>KKKGSVVIVGRINLSGDTAYAQQTRGEEGCQETSQTGRDKNQVEGEVQIVSTATQTFLATSINGVLWTVYHGAGTRTIASPKGPVTQMYTNVDKDLVGWQAPQGSRSLTPCTCGSSDLYLVTRHADVIPVRRRG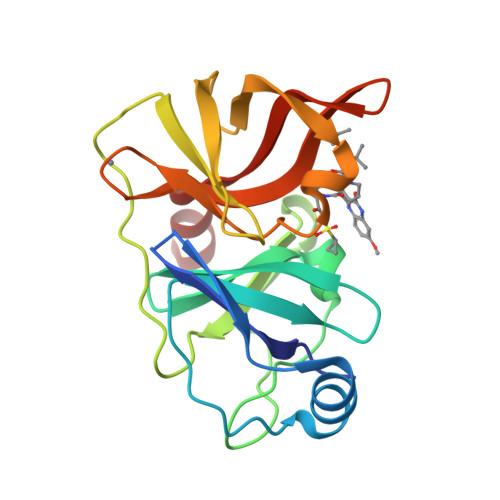DSRGSLLSPRPISYLKGSSGGPLLCPAGHAVGIFRTAVSTRGVAKAVDFIPVESLETTMR[4x]>[4x]GPAESLPDLKIEKLDEGVYVHTSFEEVNGWGVVPKHGLVVLVNAEAYLIDTPFTAKDTEKLVTWFVERGYKIKGSISSHFHSDSTGGIEWLNSRSIPTYASELTNELLKKDGKVQATN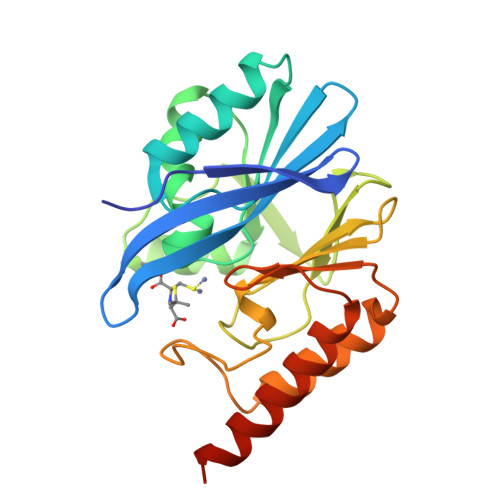SFSGVNYWLVKNKIEVFYPGPGHTPDNVVVWLPERKILFGGCFIKPYGLGNLGDANIEAWPKSAKLLKSKYGKAKLVVPSHSEVGDASLLKLTLEQAVKGLNESKKPSKPSN>RSPWARWFPKTLPCDVTLDVSKNHVIVDCTDKHLTEIPGGIPTNTTNLTLTINHIPDISPASFHRLVHLVEIDFRCNCVPIRLGSKSNMCPRRLQIKPRSFSGLTYLKSLYLDGNQLLEIPQGLPPSLQLLSLEANNIFSIRKEQLTELANIEILYLGQNCYYRNPCYVSYSIEKDAFLNLTKLKVLSLKDNNVTTVPTVLPSTLTELYLYNNMIAEIQEDDFNNLNQLQILDLSGNCPRCYNAPFPCTPCKNNSPLQIPVNAFDALTELKVLRLHSNSLQHVPPRWFKNINNLQELDLSQNFLAKEIGDAKFLHFLPNLIQLDLSFNFELQVYRASMNLSQAFSSLKSLKILRIRGYVFKELKSFQLSPLHNLQNLEVLDLGTNFIKIANLSMFKQFKRLKVIDLSVNKISPSGDSLVPRGSSNARTSVESYEPQVLEQLYYFRYDKYARSCRFKNKEASFTSVQESCYKYGQTLDLSKNSIFFIKSSDFQHLSFLKCLNLSGNLISQTLNGSEFQPLAELRYLDFSNNRLDLLHSTAFEELRKLEVLDISSNSHYFQSEGITHMLNFTKNLKVLQKLM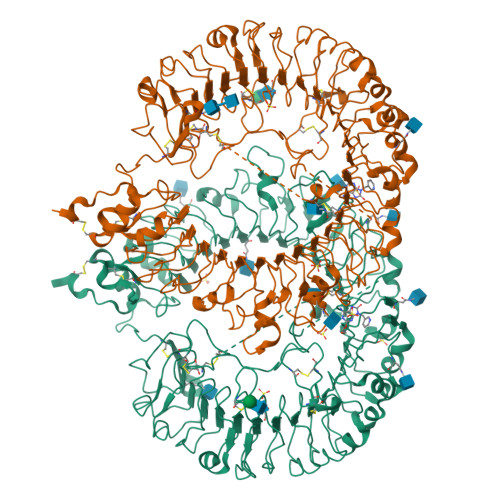MNDNDISSSTSRTMESESLRTLEFRGNHLDVLWRDGDNRYLQLFKNLLKLEELDISKNSLSFLPSGVFDGMPPNLKNLSLAKNGLKSFIWEKLRYLKNLETLDLSHNQLTTVPERLSNCSRSLKNLILKNNQIRSLTKYFLQDAFQLRYLDLSSNKIQMIQKTSFPENVLNNLKMLLLHHNRFLCTCDAVWFVWWVQHTEVTIPYLATDVTCVGPGAHKGQSVISLDLYTCELDLTNEFLVPR[2x]>[2x]MPVTLSFGNHQNYTLNESRLAHLLSADKEKAIHMGGWDKVQDHFR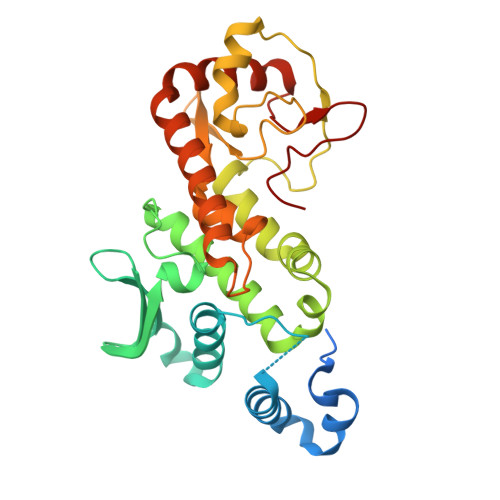AEKKDHALEVLHSIIHGQGRGEPGEMEVNVEDINKIYAFKRLQHLACPAHQDLFTIKMDASQTQFLLMVGDTVISQSNIKDILNISDDAVIESMSREERQLFLQICEVIGSKMTWHPELLQESISTLRKEVTGNAQIKTAVYEMMRPAEAPDHPLVEWQDSLTADEKSMLACINAGNFEPTTQFCKIGYQEVQGEVAFSMMHPCISYLLHSYSPFSEFKPTNSGFLKKLNQDYNDYHAKKMFIDVILEKLYLTHERSLHIGKDGCSRNILLT> MPEGPELHLASQFVNEACRALVFGGCVEKSSVSRNPEVPFESSAYRISASARGKELRLILSPLPGAQPQQEPLALVFRFGMSGSF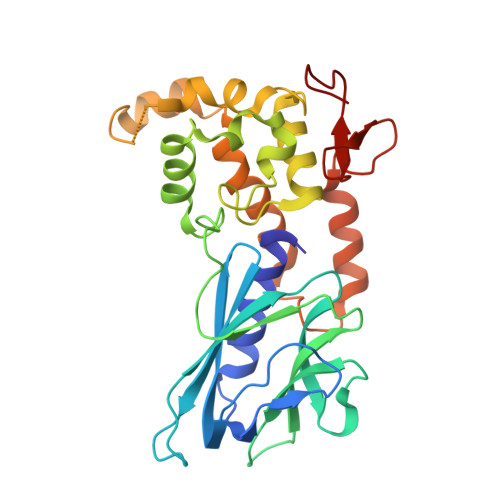QLVPREELPRHAHLRFYTAPPGPRLALCFVDIRRFGRWDLGGKWQPGRGPCVLQEYQQFRESVLRNLADKAFDRPICEALLDQRFFNGIGNYLRAEILYRLKIPPFEKARSVLEALQQHRPSPELTLSQKIRTKLQNPDLLELCHSVPKEVVQLGGRGYGSESGEEDFAAFRAWLRCYGMPGMSSLQDRHGRTIWFQGDPGPLAP> MRVDELRVDERIKSTLKERGIESFYPPQAEALKSGILEGKNALISIPTASGKTLIAEIAMVHRILTQGGKAVYIVPLKALAEEKFQEFQDWEKIGLRVAMATGDYDSKDEWLGKYDIIIATAEKFDSLLRHGSSWIKDVKILVADEIHLIGSRDRGATLEVILAHMLGKAQIIGLSATIGNPEELAEWLNAELIVSDWRPVKLRRGVFYQGFVTWEDGSIDRFSSWEELVYDAIRKKKGALIFVNMRRKAERVALELSKKVKSLLTKPEIRALNELADSLEENPTNEKLAKAIRGGVAFHHAGLGRDERVLVEENFRKGIIKAVVATPTLSAGINTPAFRVIIRDIWRYSDFGMERIPIIEVHQMLGRAGRPKYDEVGEGIIVSTSDDPREVMNHYIFGKPEKLFSQLSNESNLRSQVLALIATFGYSTVEEILKFISNTFYAYQRKDTYSLEEKIRNILYFLLENEFIEISLEDKIRPLSLGIRTAKLYIDPYTAKMFKDKMEEVVKDPNPIGIFHLISLTPDITPFNYSKREFERLEEEYYEFKDRLYFDDPYISGYDPYLERKFFRAFKTALVLLAWINEVPEGEIVEKYSVEPGDIYRIVETAEWLVYSLKEIAKVLGAYEIVDYLETLRVRVKYGIREELIPLMQLPLVGRRRARALYNSGFRSIEDISQARPEELLKIE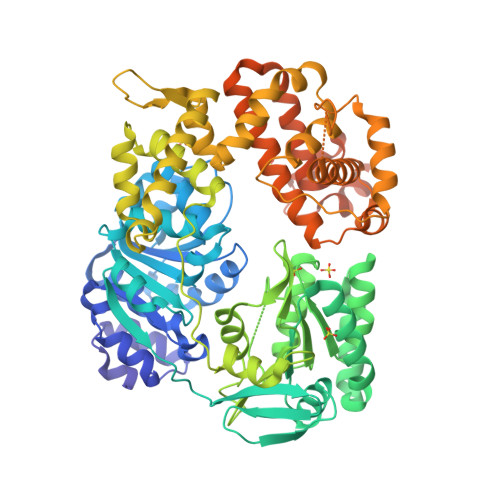GIGVKTVEAIFKFLGKNVKISEKPRKSTLDYFLKS> ADTIVAVELDTYPNTDIGDPSYPHIGIDIKSVRSKKTAKWNMQNGKVGTAHIIYNSVGKRLSAVVSYPNGDSATVSYDVDLDNVLPEWVRVGLSASTGLYKETNTILSWSFTSKLKSNSTHETNALHFMFNQFSKDQKDLILQGDATTGTEGNLRLTRVSSNGSPQGSSVGRA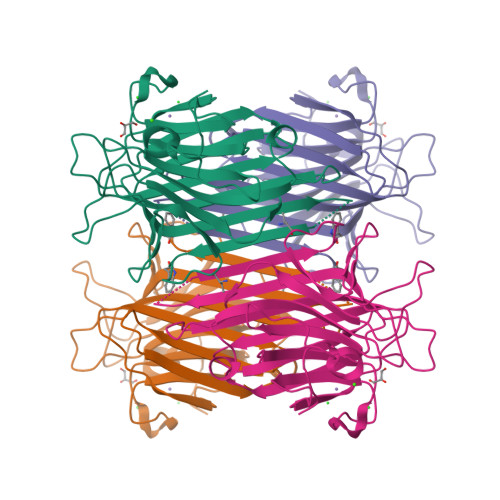LFYAPVHIWESSAVVASFEATFTFLIKSPDSHPADGIAFFISNIDSSIPSGSTGRLLGLFPDAN> ARAVIFTGNSISHEDAKKILRANYQPPVRRFQLEKFVQQGYKVIGIIDGIFFDRAAVGHREILSALNAGVKVVGGASMGALRASELDTHGMVGVGKVYEWYRDGVIESDDEVAVSTNPDTFEPISVPLVNIRETLKAALDTGLVSEKEHNALLDLAINT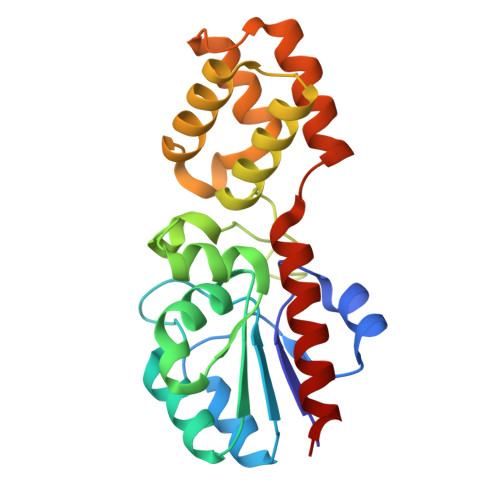YYPDRSYLGLTKEGGKKGLIPKEKGKQLLDFCLNSEVDIKRQDAVLVLETVKKLIEEA>SLEVSVGKATDIYAVNGTEILLPCTFSSCFGFEDLHFRWTYNSSDAFKILIEGTVKNEKSDPKVTLKDDDRITLVGSTKEKMNNISIVLRDLEFSD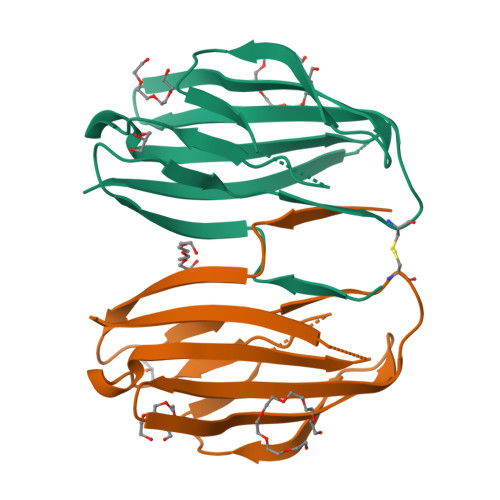TGKYTCHVKNPKENNLQHHATIFLQVV[2x]>SNAMRIGHGFDVHAFGGEGPIIIGGVRIPYEKGLLAHSDGDVALHALTDALLGAAALGDIGKLFPDTDPAFKGADSRELLREAWRRIQAKGYTLGNVDVTIIAQAPKMLPHIPQMRVFIAEDLGCHMDEVNVK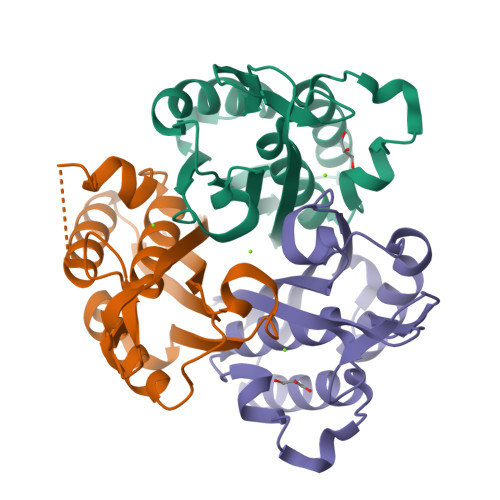ATTTEKLGFTGRGEGIACEAVALLMKAAK[3x]> IVGGKVCPKGECPWQVLLLVNGAQLCGGTLINTIWVVSAAHCFDKIKNWRNLIAVLGEHDLSEHDGDEQSRRVAQVIIPSTYVPGTTNHDIALLRLHQPVVLTDHVVPLCLPERTFSERTLAFVRFSLVSGWGQLLDRGATALELMVLNVPRLMTQDCLQQSRKVGDSPNITEYMFCAGYSDGSKDSCKGDSGGPHATH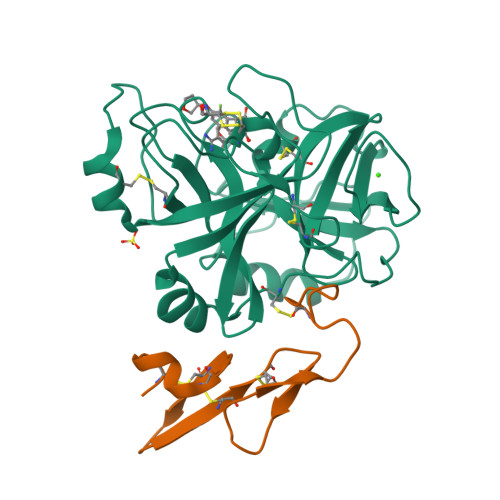YRGTWYLTGIVSWGQGCATVGHFGVYTRVSQYIEWLQKLMRSEPRPGVLLRAPFP;> ICVNENGGCEQYCSDHTGTKRSCRCHEGYSLLADGVSCTPTVEYPCGKIPILE>MAYAQWVIIIIHNVGSQDVKIKNLKASWGKLHADGDKDAEVSASNYEGKIVKPDEKLQINASGRSDAAAGTTGTFDLVDPADGDKQVRHFYWDSPWGSKTNTWTVSGSNTKWMIEYSGQNLDSGALGTITVDTLKKGENLYFQ[4x];>[2x]HHHHHHHHSQAGDTLNDVIQDPTRRNKLINDNNLLKGIIMGRDGPVPSSRELIVRPDTLRAIINNRATIETTTMEAEFTETLMESNYNSASVKVSAPFITANSEYSESSSFKNTE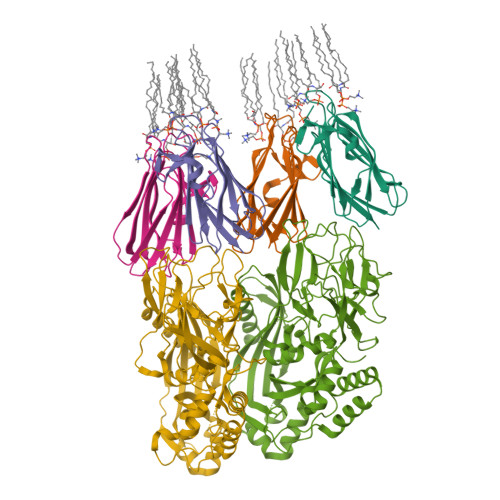TEKSMYTSSRYLFPQGRIDFTTPDSGFDDVIKLSPQFTSGVQAALAKATGTEKREALQNLFQEYGHVFRTKVHIGGVLSAHTMETFSRSENETEVKQDVKAGLEGAVKGWGGGATAGHGNTQGTITTSQNRKLNVKYIVNVVDYTKIQNTEEWVASTNQSEHWRVIEVTEVTAVADLLPQPIRGQVKDLLKPLLGKWVDVEKVPGLESLPVSVYRPKGAIPAGWFWLGDTADASKALLVKPTLPARSGRNPALTSLHQGSGMTEQPFVDLPQYQYLSTYFGSFAHDTPPGSTLRGLRPDHVLPGRYEMHGDTISTAVYVTRPVDVPFPEDECFDLKSLVRVKLPGSGNPPKPRSALKKSMVLFDSGEK4-[2-[(2~{S})-2-(2-cyclopropylphenyl)pyrrolidin-1-yl]-7-azaspiro[3.5]nonan-7-yl]-~{N}-[3-nitro-4-(oxan-4-ylmethylamino)phenyl]sulfonyl-2-(1~{H}-pyrrolo[2,3-b]pyridin-5-yloxy)benzamide 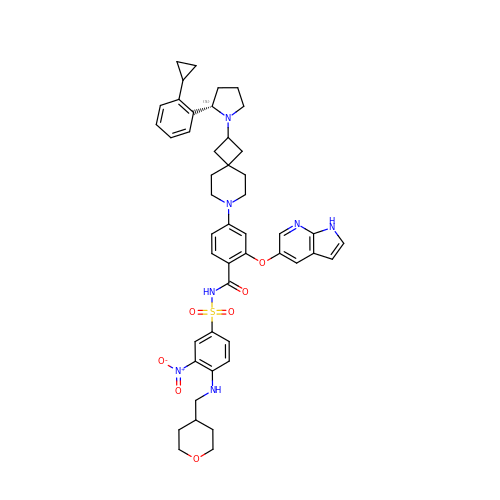| C47 H53 N7 O7 S | IVXFXSGHRVGVIZ-WBCKFURZSA-N> MAIHTCFSLIPSSFSSPKLPYPKNTTFQSPIPKLSRPTFMFDRKGSFQNGTAAVPAVGEDFPIDYADWLPKRDPNDRRRAGILLHPTSFPGPYGIGDLGPQAFKFLDWLHLAGCSLWQVLPLVPPGKRGNEDGSPYSGQDANCGNTLLISLEELVDDGLLKMEELPEPLPTDRVNYSTISEIKDPLITKAAKRLLSSEGELKDQLENFRRDPNISSWLEDAAYFAAIDNSVNTISWYDWPEPLKNRHLAALEEVYQSEKDFIDIFIAQQFLFQRQWKKVRDYARSKGISIMGDMPIYVGYHSADVWANKKQFLLNRKGFPLIVSGVPPDAFSETGQLWGSPLYDWKAMEKDGFSWWVRRIQRATDLFDEFRIDHFRGFAGFWAVPSEEKIAILGRWKVGPGKPLFDAILQAVGKINIIAEDLGVITEDVVQLRKSIEAPGMAVLQFAFGSDAENPHLPHNHEQNQVVYTGTHDNDTIRGWWDTLPQEEKSNVLKYLSNIEEEEISRGLIEGAVSSVARIAIIPMQ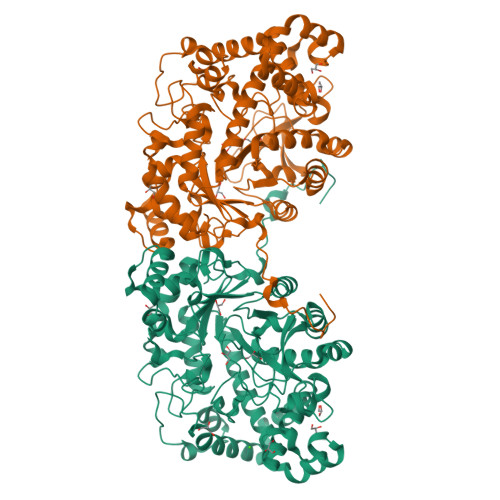DVLGLGSDSRMNIPATQFGNWSWRIPSSTSFDNLDAEAKKLRDILATYGRL> VYWDLDIQTNAVIRERAPADHLPPHPEIELQRAQLTTKLRQHYHELCSQREGIE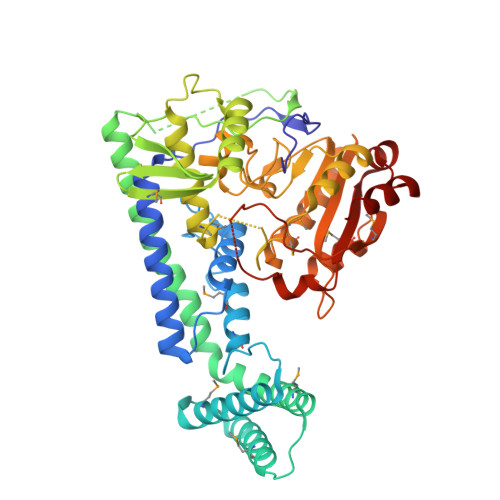PPRESFNRWLLERKVVDKGLDPLLPSECDPVISPSMFREIMNDIPIRLSRIKYKEEARKLLFKYAEAAKKMIDSRNVTPESRKVVKWNVEDTMNWLRRDHSASKEDYMDRLENLRKQCGPHVASVAKDSVEGICSKIYHISAEYVRRIRQAHLTLLKECNISVDGTESAEVQDRLVYCYPVRLSIPAPPQTRVELHFENDIACLRFKGEMVKVSRGHFNKLELLYRYSCIDDPRFEKFLSRVWCLIKRYQVMFGSGVNEGSGLQGSLPVPVFEALNKQFGVTFECFASPLNCYFKQFCSAFPDIDGFFGSRGPFLSFSPASGSFEANPPFCEELMDAMVTHFEDLLGRSSEPLSFIIFVPEWRDPPTPALTRMEASRFRRHQMTVPAFEHEYRSGSQHICKREEIYYKAIHGTAVIFLQNNAGFAKWEPTTERIQELLAAYK The protein, termed Pa Dps, adopts the Dps subunit fold and oligomerizes into a nearly spherical 12-mer quaternary structure at pH 6.0 or in the presence of divalent cations at neutral pH and above. The 12-Mer Pa Dps contains two di-iron centers at the interface of each subunit dimer, coordinated by conserved His, Glu, and Asp residues. In vitro, the di-iron centers catalyze the oxidation of Fe2+ utilizing H2O2 (not O2) as an oxidant, suggesting Pa Dps functions to aid P. aeruginosa to survive H2O2-mediated oxidative stress. The Pa Dps structure harbors a novel network of Tyr residues at the interface of each subunit dimer between the two di-iron centers, which captures radicals generated during Fe2+ oxidation at the ferroxidase centers and forms di-tyrosine linkages, thus effectively trapping the radicals within the Dps shell.

The Na+ occupies the same site as Fe1 in the di-Fe center of the Dps-c-Fe and Dps-o-Fe structures, which is coordinated by the same three ligands. In comparison, Fe2 is coordinated by only two protein-provided ligands, H49 and E68. Consequently, we hypothesized that the “Fe1-site” might have a higher propensity to bind metal ions and therefore contribute to stabilizing the subunit dimer and possibly the dodecameric structure. To test this idea, we crystallized Pa Dps from a solution containing 0.5 mM MnCl2 (Dps-c-Mn). The Dps-c-Mn structure is nearly identical to the Dps-c-Fe structure (RMSD = 0.40 Å, 1834 residues). Inspection of the ferroxidase center ligands shows an Mn atom coordinated by H37, D64, and E68, occupying the same site as Fe1 in the Dps-c-Fe and Dps-o-Fe structures and Na in the Dps-o structure. These findings support the idea that the “Fe-1” site exhibits a higher propensity to coordinate metal ions than Fe2.

>[16x]MEINIGIGEQDRAAIAEGLSRLLADTYTLYLKTHNFHWNVTGPMFNTLHLMFEGQYTELAVAVDDIAERIRALGFPAPGTYAAYARLSSIKEEEGVPEAEEMIRQLVQGQEAVVRTARSIFPLLDKVSDEPTADLLTQRMQVHEKTAWMLRSLLAS>DTGPTGIKYDLDRHQYNYVDAVCYENRLHWFAKYFPYLVLLHTLIFLACSNFWFKFPRTSSKLEHFVSILLKCFDSPWTTRALSETVVEESDPKPAFSKMNGSMDKKSSTVSEDVEATVPMLQRTKSRIEQGIVDRSETGVLDKKEGEQAKALFEKVKKFRTHVEEGDIVYRLYMRQTIIKVIKFALIICYTVYYVHNIKFDVDCTVDIESLTGYRTYRCAHPLATLFKILASFYISLVIFYGLICMYTLWWMLRRSLKKYSFESIREESSYSDIPDVKNDFAFMLHLIDQYDPLYSKRFAVFLSEVSENKLRQLNLNNEWTLDKLRQRLTKNAQDKLELHLFMLSGIPDTVFDLVELEVLKLELIPDVTIPPSIAQLTGLKELWLYHTAAKIEAPALAFLRENLRALHIKFTDIKEIPLWIYSLKTLEELHLTGNLSAENNRYIVIDGLRELKRLKVLRLKSNLSKLPQVVTDVGVHLQKLSINNEGTKLIVLNSLKKMVNLTELELIRCDLERIPHSIFSLHNLQEIDLKDNNLKTIEEIISFQHLHRLTCLKLWYNHIAYIPIQIGNLTNLERLYLNRNKIEKIPTQLFYCRKLRYLDLSHNNLTFLPADIGLLQNLQNLAVTANRIEALPPELFQCRKLRALHLGNNVLQSLPSRVGELTNLTQIELRGNRLECLPVELGECPLLKRSGLVVEEDLFSTLPPEVKERLWRADKEQASNSLEVLFQ[2x];> MIPVTEFRQFSEQQPAFRVLKPWWDVFTDYLSVAMLMIGVFGCTLQVMQDKIICLPKRVQPAQNHSSVPNVSQAVISTTPLPPPKPSPTNPATVEMKGLKTDLDLQQYSFINQMCYERALHWYAKYFPYLVLIHTLVFMLCSNFWFKFPGSSSKIEHFISILGKCFDSPWTTRALSEVSGEDSEEKDNRKNNMNRSGTIQSGPEGNLVRSQSLKSIPEKFVVDKSAAGALDKKEGEQAKALFEKVKKFRLHVEEGDILYAMYVRQTVLKVIKFLIIIAYNSALVSKVQFTVDCNVDIQDMTGYKNFSCNHTMAHLFSKLSFCYLCFVSIYGLTCLYTLYWLFYRSLREYSFEYVRQETGIDDIPDVKNDFAFMLHMIDQYDPLYSKRFAVFLSEVSENKLKQLNLNNEWTPDKLRQKLQTNAHNRLELPLIMLSGLPDTVFEITELQSLKLEIIKNVMIPATIAQLDNLQELCLHQCSVKIHSAALSFLKENLKVLSVKFDDMRELPPWMYGLRNLEELYLVGSLSHDISKNVTLESLRDLKSLKILSIKSNVSKIPQAVVDVSSHLQKMCVHNDGTKLVMLNNLKKMTNLTELELVHCDLERIPHAVFSLLSLQELDLKENNLKSIEEIVSFQHLRKLTVLKLWYNSIAYIPEHIKKLTSLERLFFSHNKVEVLPSHLFLCNKIRYLDLSYNDIRFIPPEIGVLQSLQYFSITCNKVESLPDELYFCKKLKTLKIGKNSLSVLSPKIGNLLFLSYLDIKGNHFEVLPPELGDCRALKRAGLVVEDALFETLPSDVREQMK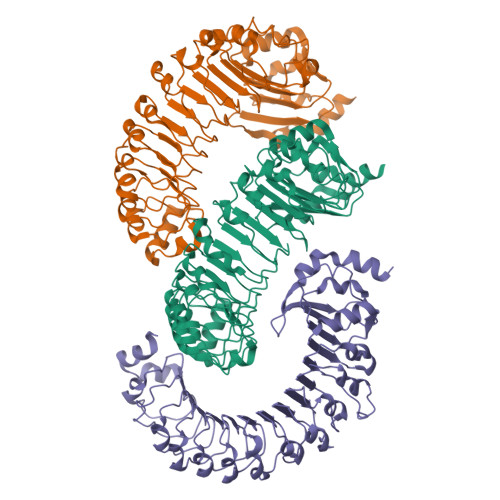ADSNSENLYFQG>MSIKIRDFGLGSDLISLTNKAGVTISFTNLGARIVDWQKDGKHLILGFDSAKEYLEKDAYPGATVGPTAGRIKDGLVKISGKDYILNQNEGPQTLHGGEESIHTKLWTYEVTDLGAEVQVKFSLVSNDGTNGYPGKIEMSVTHSFDDDNKWKIHYEAISDKDTVFNPTGHVYFNLNGDASESVENHGLRLAASRFVPLKDQTEIVRGDIVDIKNTDLDFRQEKQLSNAFNSNMEQVQLVKGIDHPFLLDQLGLDK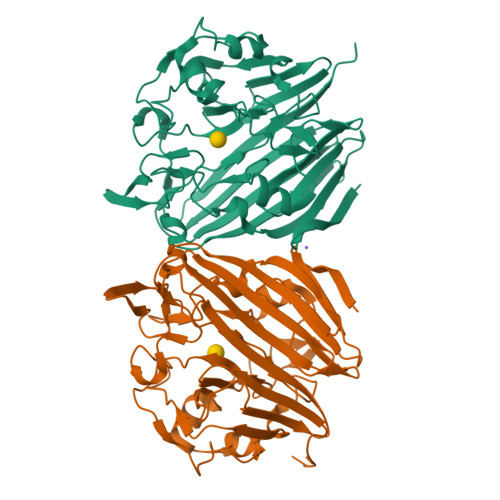EQARLTLDDTSISVFTDQPSIVIFTANFGDLGTLYHEKKQVHHGGITFQCQVSPGSEQIPELGDISLKAGEKYQATTIYSLHTKLEHHHHHH[2x]>MGHHHHHHGSHMSQNVYIVSTARTPIGSFQGSLSSKTAVELGAVALKGALAKVPELDASKDFDEIIFGNVLSANLGQAPARQVALAAGLSNHIVASTVNKVCASAMKAIILGAQSIKCGNADVVVAGGCESMTNAPYYMPAARAGAKFGQTVLVDGVERDGLNDAYDGLAMGVHAEKCARDWDITREQQDNFAIESYQKSQKSQKEGKFDNEIVPVTIKGFRGKPDTQVTKDEEPARLHVEKLRSARTVFQKENGTVTAANASPINDGAAAVILVSEKVLKEKNLKPLAI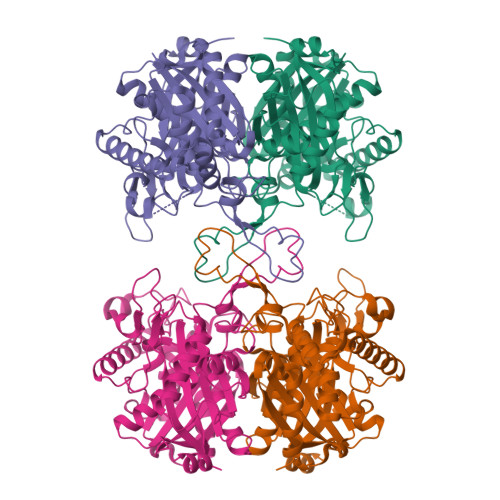IKGWGEAAHQPADFTWAPSLAVPKALKHAGIEDINSVDYFEFNEAFSVVGLVNTKILKLDPSKVNVYGGAVALGHPLGCSGARVVVTLLSILQQEGGKIGVAAICNGGGGASSIVIEKI[2x]>SATLTAKNLAKAYKGRRVVEDVSLTVNSGEIVGLLGPNGAGKTTTFYMVVGIVPRDAGNIIIDDDDISLLPLHARARRGIGYLPQEASIFRRLSVYDNLMAVLQIRDDLSAEQREDRANELMEEFHIEHLRDSMGQSLSGGERRRVEIARALAANPKFILLDQPFAGVDPISVIDIKRIIEHLRDSGLGVLITDHNVRETLAVCERAYIVSQGHLIAHGTPTEILQDEHVKRVYLGEDFRL[2x]

The LptB2FGC exporter is an essential ABC transporter that assembles lipopolysaccharides (LPS) on the surface of Gram-negative bacteria to form a permeability barrier against many antibiotics. LptB2FGC extracts newly synthesized LPS molecules from the inner membrane and powers their transport across the periplasm and through the outer membrane. Like other ABC transporters, LptB2FGC contains two nucleotide-binding domains (NBDs; LptB2) that function as a single ATPase that interacts with and powers two transmembrane domains (TMDs; LptF and LptG), which transport the LPS substrate. Here, we discovered a novel C-terminal domain (CTD) in LptB that is crucial for LPS transport in Escherichia coli.

Therefore, to gain structural insight into the role of the wild-type CTD of LptB, we attempted to crystallize ADP- and ATP-bound E. coli LptB proteins with N-terminal His tags after confirming that they do not affect function. To trap the ATP-bound form, we used the catalytically dead LptBE163Q protein as was done with CT-tagged LptBE163Q-EHis8 as previously described. We did not obtain a structure of ADP-bound His8-LptB, but we solved a 1.96-Å structure of ATP-bound His8-LptBE163Q. The new structure resembled that of LptBE163Q-EHis8, except that it included a fully resolved CTD. The CTD is located at the LptB dimer interface below the ATP-binding sites, and it consists of a short helix (residues V230 to L235) followed by a turn and a loop (residues G236 to L241). Within each LptB monomer, CTD-helix residue Y234 interacts with Walker-A invariant residue G36 and residue P37. In addition, CTD-helix residue L235 forms van der Waal interactions with CTD-loop residue F239. The new ATP-bound structure also revealed a functional interaction between the carboxylate of CTD-loop residue L241, which is the last residue of LptB, and residue R198 from both monomers. Residue R198 is located in the switch helix that follows the switch motif (or H loop).>[2x]TMAHHHHHHVTNSTDGRADGRLRVVVLGSTGSIGTQALQVIADNPDRFEVVGLAAGGAHLDTLLRQRAQTGVTNIAVADEHAAQRVGDIPYHGSDAATRLVEQTEADVVLNALVGALGLRPTLAALKTGARLALANKESLVAGGSLVLRAARPGQIVPVNSEHSALAQCLRGGTPDEVAKLVLTASGGPFRGWSAADLEHVTPEQA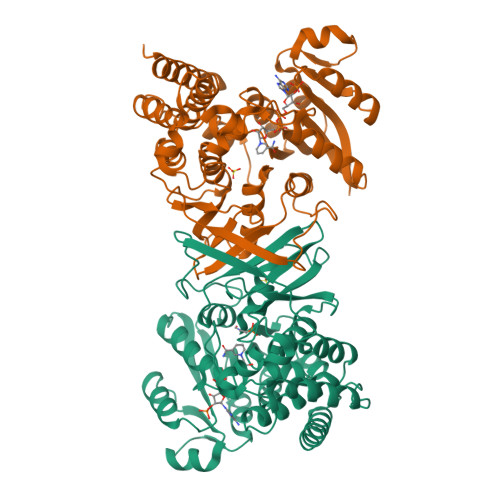GAHPTWSMGPMNTLNSASLVNKGLQVIETHLLFGIPYDRIDVVVHPQSIIHSMVTFIDGSTIAQASPPDMKLPISLALGWPRRVSGAAAACDFHTASSWEFEPLDTDVFPAVELARQAGVAGGCMTAVYNAANEEAAAAFLAGRIGFPAIVGIIADVLHAADQWAVEPATVDDVLDAQRWARERAQRAVSGM>QVVQVNDSMYGFIGTDVVLHCSFANPLPSVKITQVTWQKASNGSKQNMAIYNPTMGVSVLPPYEKRVEFLRPSFIDGTIRLSG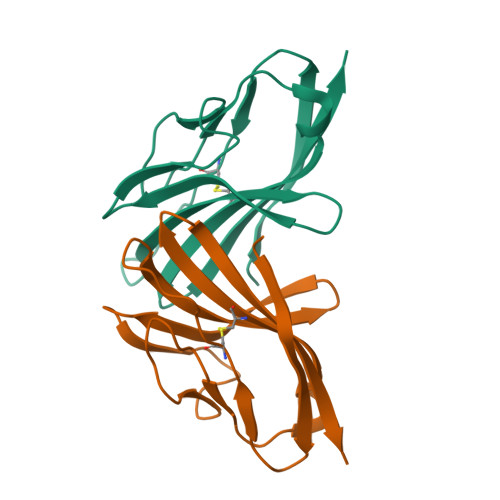LELEDEGMYICEFATFPTGNRESQLNLTVMA[2x]>[4x]MSLALNPAVAPIKSI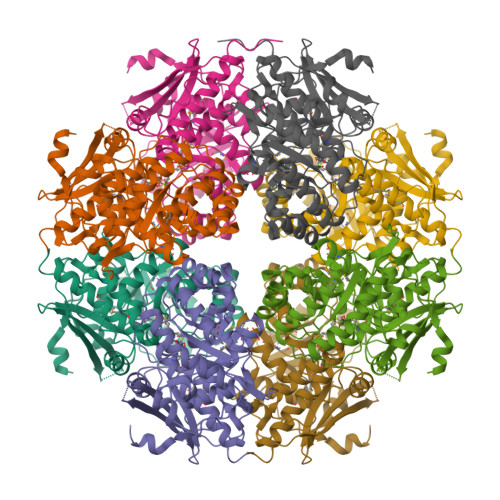EFIPVNYQASNWSQNTVVVKVTDENGVYGLGEADGSPDAILAYANIETEHKWLTNITEKAIGRLPIEINAIWDAMYDATQWQGMRGLGMFALSGIDMALYDLAGKQLGVPAYQLLGGTNKDKVHPYLTLYPAIPVDASLDVAIKGYAPLLEKAKAHNIRAVKVCVPIKADWSTKEVAYYLRELRGILGHDTDMMVDYLYRFTDWYEVARLLNSIEDLELYFAEATLQHDDLSGHAKLVENTRSRICGAEMSTTRFEAEEWITKGKVHLLQSDYNRCGGLTELRRITEMATANNVQVMPHNWKTGITSAAAIHYQFAVGNAPYFEYVHPEFCDGELRKYLVTPEAELVDGGFAKPTAPGLGIDLNQEFLASLEGHHHHHH> MDLTNGGVSPAATSAPLDWTTFRRVFLIDDAWRPLMEPELANPLTAHLLAEYNRRCQTEEVLPPREDVFSWTRYCTPDEVRVVIIGQDPYHHPGQAHGLAFSVRANVPPPPSLRNVLAAVKNCYPEARMSGHGCLEKWARDGVLLLNTTLTVKRGAAASHSRIGWDRFVGGVIRRLAARRPGLVFMLWGTHAQNAIRPDPRVHCVLKFSHPSPLSKVPFGTCQHF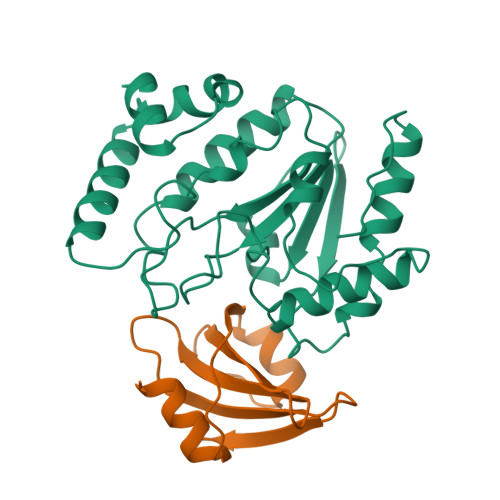LVANRYLETRSISPIDWSV;> TNLSDIIEKETGKQLVIQESILMLPEEVEEVIGNKPESDILVHTAYDESTDENVMLLTSDAPEYKPWALVIQDSNGENKIKML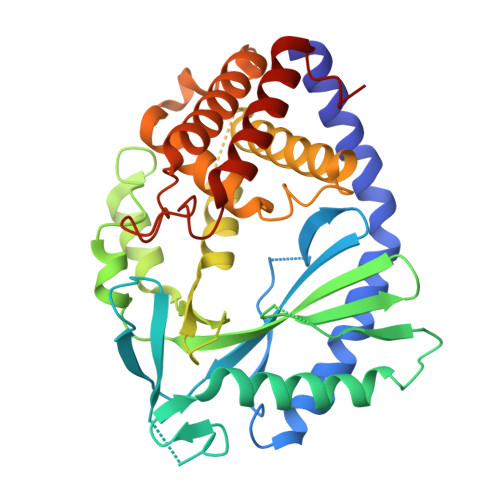>[2x]GSGASKLRAVLEKLKLSRDDISTAAGMVKGVVDHLLLRLKCDSAFRGVGLLNTGSYYEHVKISAPNEFDVMFKLEVPRIQLEEYSNTRAYYFVKFKRNPKENPLSQFLEGEILSASKMLSKFRKIIKEEINDIKDTDVIMKRKRGGSPAVTLLISEKISVDITLALESKSSWPASTQEGLRIQNWLSAKVRKQLRLKPFYLVPKHAKEGNGFQEETWRLSFSHIEKEILNNHGKSKTCCENKEEKCCRKDCLKLMKYLLEQLKERFKDKKHLDKFSSYHVKTAFFHVCTQNPQDSQWDRKDLGLCFDNCVTYFLQCLRTEKLENYFIPEFNLFSSNLIDKRSKEFLTKQIEYERNNEFPVFDEF4-[3-amino-6-(3-hydroxyphenyl)pyrazin-2-yl]benzoic acid | C17 H13 N3 O3 | 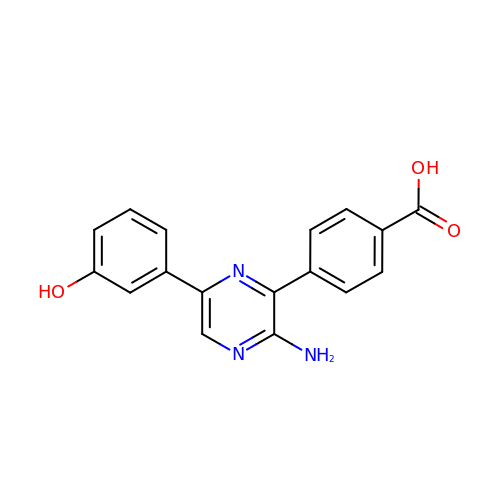SMCZWNHNLRIBBG-UHFFFAOYSA-N> APEITEEMEKEIKNVFRNGNQDEVLSEAFRLTITRKDIQTLNHLNWLNDEIINFYMNMLMERSKEKGLPSV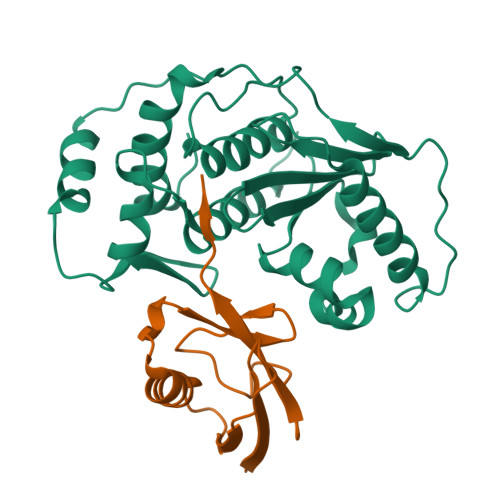HAFNTFFFTKLKTAGYQAVKRWTKKVDVFSVDILLVPIHLGVHWCLAVVDFRKKNITYYDSMGGINNEACRILLQYLKQESIDKKRKEFDTNGWQLFSKKSQIPQQMNGSDCGMFACKYADCITKDRPINFTQQHMPYFRKRMVWEILHRKLL;> DHINLKVAGQDGSVVQFKIKRHTPLSKLMKAYCERQGLSMRQIRFRFDGQPINETDTPAQLEMEDEDTIDVFQQQTGG Gram-positive bacteria, including the common wound-infecting Staphylococcus aureus, the virulent food-borne pathogen Listeria monocytogenes, and Streptococcus pneumoniae that causes pneumonia, utilize cholesterol-dependent cytolysins (CDCs) to attack and kill mammalian and human cells. The bacteria produce and release CDCs as water-soluble monomers that attach to cholesterol-containing cell membranes, where they assemble into large, 200–500 Å cytolytic pores. X-ray structures of pneumolysin (PLY) from S. pneumoniae show that the soluble toxin monomers are roughly rod-shaped and consist of four domains (D1-D4). Sequence comparison suggests that all CDCs have the same domain structure and therefore insert into target membranes in essentially the same way.

To understand the functional role of individual sidechains in oligomerization, prepore and pore formation, we mutated Asp168 that, as the structure suggests, might be involved in forming a salt bridge between adjacent subunits to alanine (PLYD168A). X-ray data were collected to 2.45 and 2.5 Å resolution from crystals of PLYD168A and PLYΔ146/147. Superposition of both structures on PLYWT showed no significant overall differences, although a detailed comparison indicated small changes in domain D2, helix bundle HB2 and in two of the D4 loops. Around the mutated residue in PLYD168A differences were restricted to sidechain orientations, while the deletion of two residues in PLYΔ146/147 caused significant conformational changes in the loop connecting helix α5 to strand β7 of the central β-sheet. (B) In the pore complex, Asp168 near the end of one long trans-membrane β-hairpin (HP1) forms a salt bridge with Lys271 in the other trans-membrane β-hairpin (HP2) of the adjacent monomer. Like PLYWT, PLYD168A bound to cholesterol-containing liposomes and oligomerized into rings. However, unlike PLYWT that lysed the liposomes within a short time, liposomes incubated with PLYD168A remained intact for hours. Frequently, the rings detached from the liposomes, indicating they were prepores that had not yet inserted into the membrane. This is also reflected by the hemolytic activity, which was reduced by 80% compared to PLYWT, highlighting the important role of Asp168 in ionic interactions between β-strands that stabilize the pore complex. The detachment of PLYD168A rings indicates that the mutant does not insert into the membrane as easily as PLYWT to form pores.

>AHHHHHHSSGLVPRGSHMANKAVNDFILAMNYDKKKLLTHQGESIENRFIKEGNQLPDEFVVIERKKRSLSTNTSDISVTATNDSRLYPGALLVVDETLLENNPTLLAVDRAPMTYSIDLPGLASSDSFLQVEDPSNSSVRGAVNDLLAKWHQDYGQVNNVPARMQYEKITAHSMEQLKVKFGSAFEKTGNSLDIDFNSVHSGEKQIQIVNFKQIYYTVSVDAVKNPGDVFQDTVTVEDLKQRGISAERPLVYISSVAYGRQVYLKLETTSKSDEVEAAFEALIKGVKVAPQTEWKQILDNTEVKAVILGGDPSSGARVVTGKVDMVEDLIQEGSRFTADHPGLPISYTTSFLRDNVVATFQNSTDYVETKVTAYRNGDLLLDHSGAYVAQYYITWDELSYDHQGKEVLTPKAWDRNGQDLTAHFTTSIPLKGNVRNLSVKIRECTGLAWEWWRTVYEKTDLPLVRKRTISIWGTTLYPQVEDKVEND[2x]>MSQAIGILELRSIAAGMELGDAMLKSANVDLLVSKTISRGKFLLMLGGDIGAIQQA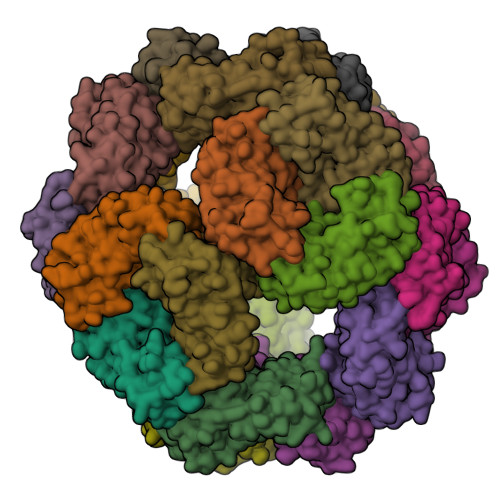IETGTSQAGRLLVDSLVLANIHPSVLPAISGLNSVDKRQAVGIVETRSVAACISAADRAVKGSNVTLVRVHMARGIGGKCYMVVAGDVSDVALAVTVASSSAGAYGRLVYASLIPRPHEAMWRQMVEGLEHHHHHH[8x]>[2x]MGSDKIHHHHHHMKISPLCPSCLLGRVYYEAKLVTDDEDLISQCVDESLKILAENYSSRPINAHLAT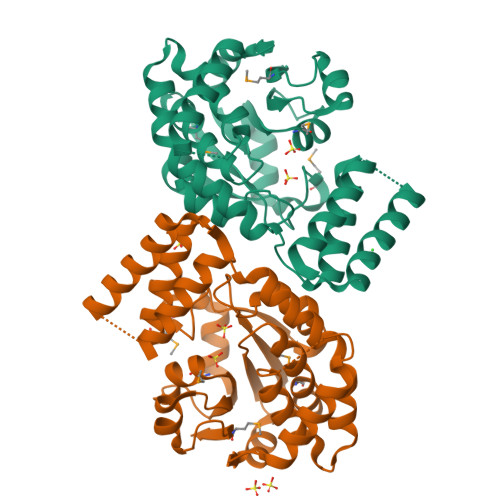RIHRRVYEILGVEDPYAEVKARANEVARQVLPLAKEIVEGSDDPFKTAVIVSIVGNNFDYGVQGHKVVEEEFRDFLKRKVQEGLKINDTERIKELSSGKVVYLTDNAGEIFFDTLLMKEIKRRCEKLTAVVRGRPIISDATIEDARLARVDKIADELLTNGKGAIGIIMDELPDETRKALEEADLIVAKGMANYECLSDGSLKPIAFLLTAKCEPVARDIGVNVGDMVAKVVE> MATKAARVPRTVLPFEAMPRRPGNRRNRLNQIRREQGYEDLHLEVHQTFQELGPIFRYDLGGAGMVCVMLPEDVEKLQQVDSLHPHRMSLEPWVAYRQHRGHKCGVFLLNGPEWRFNRLRLNPEVLSPNAVQRFLPMVDAVARDFSQALKKKVLQNARGSLTLDVQPSIFHYTIEASNLALFGERLGLVGHSPSSASLNFLHALEVMFKSTVQLMFMPRSNSRNTSPKVWKEHFEAWDCIFQYGDNCIQKIYQELAFSRPQQYTSIVAELLLNAELSPDAIKANSMELTAGSVDTTVFPLLMTLFELARNPNVQQALRQESLAAAASISEHPQKATTELPLLRAALKETLRLYPVGLFLERVASSDLVLQNYHIPAGTLVRVFLYSLGRNPALFPRPERYNPQRWLDIRGSGRNFYHVPFGFGMRQCLGRRLAEAEMLLLLHHVLKHLQVETLTQEDIKMVYSFILRPSMFPLLTFRAINHHHHHH

Human cytochromes P45011β (CYP11B1) and P450aldo (CYP11B2) are monooxygenases that synthesize cortisol through steroid 11β-hydroxylation and aldosterone through a three-step process comprising 11β-hydroxylation and two 18-hydroxylations, respectively. The last step of the synthetic pathway of the major glucocorticoids, cortisol in human and corticosterone in rodents, is catalyzed by steroid 11β-hydroxylase cytochrome P45011β (CYP11B1), while those of the potent mineralocorticoid, aldosterone, are catalyzed by aldosterone synthase cytochrome P450aldo (CYP11B2). They are a pair of closely-related cytochromes P450, and their amino acid sequences of the mature enzymes share 94% identities to each other. As their physiological functions, CYP11B1 converts 11-deoxycortisol (DOF) and 11-deoxycorticosterone (DOC) to cortisol and corticosterone, respectively, while CYP11B2 catalyzes, in addition to 11β-hydroxylation of DOC, 18-hydroxylation and 18-oxidation to yield aldosterone. Thus, the key feature differentiating between the two enzymes is the capability to process the successive 18-hydroxylation following 11β-hydroxylation.

The mutant is generated in our attempt to increase in protein hydrophilicity for crystallography by replacing hydrophobic residues with hydrophilic ones at six positions on the distal surface putatively associating with mitochondrial membranes (residues in red). The crystal structure of the CYP11B1 mutant complexed with metyrapone was determined at a resolution of 1.4 ​Å. The asymmetric unit of the crystals has a single protein molecule, and two molecules of cholate are co-crystallized exposing their β-face to solvent. The nitrogen atom in 2-pyridinyl of metyrapone coordinates to the heme iron, being consistent with the low-spin state. The other nitrogen atom in 1-pyridinyl seems to interact with a water molecule which forms hydrogen bonds to a propionate of the heme and the main chain amide nitrogen of E383. First, the amino acid replacements at the four residues (W49R, L50N, L53N, and W56R) in helix A′ of the wild type caused a shift of the helix together with a shift of the turn from β1-1 to β1-2. Second, the replacements at the two residues (L244N and W247N) in helix G′ of the wild type caused uncoiling in part and a shift of it. Along with the structural shifts, the substrate access channel has an open entrance. The surface representations delineate differences in geometry among them. The innermost space, which is formed by the residues including W116, R120, F130, and E310, is reduced in the mutant compared to the CYP11B1 wild type (Fig. 5c vs d, green boxes), whereas CYP11B2 has an enlarged space which surrounds the C3 carbonyl side of DOC. Therefore, the replacement of the amino acid residues caused a complete lack of the activity of 11β,18-dihydroxylase without marked effect on the two monohydroxylase activities.> MENTENSVDSKSIKNLEPKIIHGSESMDSGISLDNSYKMDYPEMGLCIIINNKNFHKSTGMTSRSGTDVDAANLRETFRNLKYEVRNKNDLTREEIVELMRDVSKEDHSKRSSFVCVLLSHGEEGIIFGTNGPVDLKKITNFFRGDRCRSLTGKPKLFIIQACRGTELDCGIETDSGVDDDMACHKIPVEADFL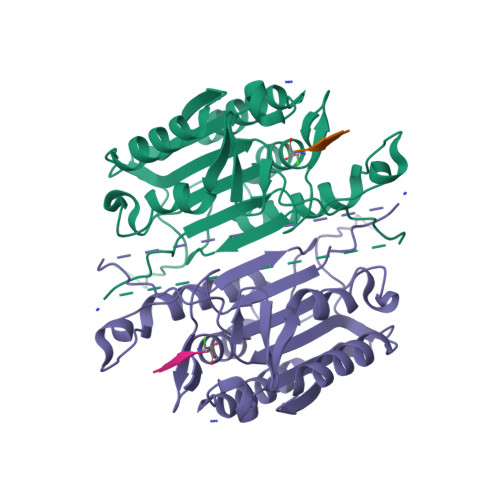YAYSTAPGYYSWRNSKDGSWFIQSLCAMLKQYADKLEFMHILTRVNRKVATEFESFSFDATFHAKKQIPCIMSMLTKELYFYHH(2R)-3-[2-(aminomethyl)-3-azanyl-1-[4-[2-(2-chloranylethanoylamino)ethylcarbamoyl]phenyl]prop-1-enyl]sulfanyl-2-(carboxyamino)propanoic 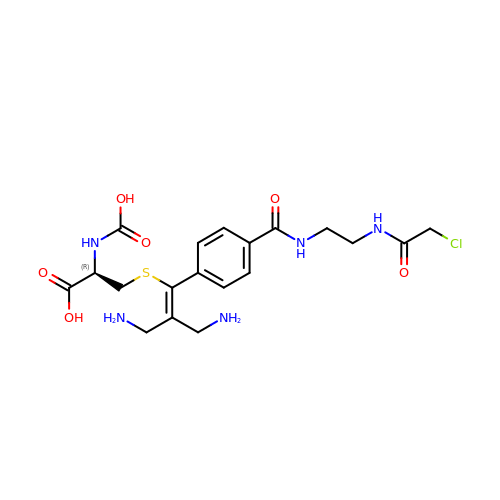acid | C19 H26 Cl N5 O6 S | SHRIZMDECXYRNC-UHFFFAOYSA-N>MQEPLAAGAVILRRFAFNAAEQLIRDINDVASQSPFRQMVTPGGYTMSVAMTNCGHLGWTTHRQGYLYSPIDPQTNKPWPAMPQSFHNLCQRAATAAGYP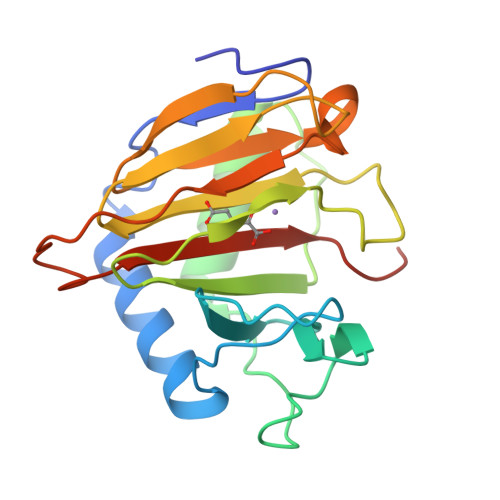DFQPDACLINRYAPGAKLSLHQDKDEPDLRAPIVSVSLGLPAIFQFGGLKRNDPLKRLLLEHGDVVVWGGESRLFYHGIQPLKAGFHPLTIDCRYNLTFRQAGKKENLYFQ[2x]>[4x]MTKYSESYCDVLIVGAGPAGLMAARVLSEYVRQKPDLKVRIIDKRSTKVYNGQADGLQCRTLESLKNLGLADKILSEANDMSTIALYNPDENGHIRRTDRIPDTLPGISRYHQVVLHQGRIERRILDSIAEISDTRIKVERPLIPEKMEIDSSKAEDPEAYPVTMTLRYMSEDESTPLQFGHKTENGLFRSNLQTQEEEDANYRLPEGKEAGEIETVHCKYVIGCDGGHSWVRRTLGFEMIGEQTDYIWGVLDAVPASNFPDIRSRCAIHSAESGSIMIIPRENNLVRFYVQLQARAEKGGRVDRTKFTPEVVIANAKKIFHPYTF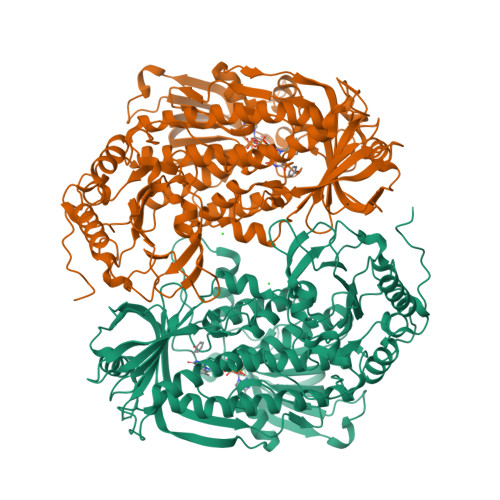DVQQLDWFTAYHIGQRVTEKFSKDERVFIAGDACHTHSPKAGQGMNTSMMDTYNLGWKLGLVLTGRAKRDILKTYEEERQPFAQALIDFDHQFSRLFSGRPAKDVADEMGVSMDVFKEAFVKGNEFASGTAINYDENLVTDKKSSKQELAKNCVVGTRFKSQPVVRHSEGLWMHFGDRLVTDGRFRIIVFAGKATDATQMSRIKKFAAYLDSENSVISRYTPKGADRNSRIDVITIHSCHRDDIEMHDFPAPALHPKWQYDFIYADCDSWHHPHPKSYQAWGVDETKGAVVVVRPDGYTSLVTDLEGTAEIDRYFSGILVEPKEKSGAQTEADWTKSTA>MMVISEKVRKALNDQLNREIYSSYLYLSMATYFDAEGFKGFAHWMKKQAQEELTHAMKFYEYIYERGGRVELEAIEKPPSNWNGIKDAFEAALKHEEFVTQSIYNILELASEEKDHATVSFLKWFVDEQVEEEDQVREILDLLEKANGQMSVIFQLDRYLGQRE[8x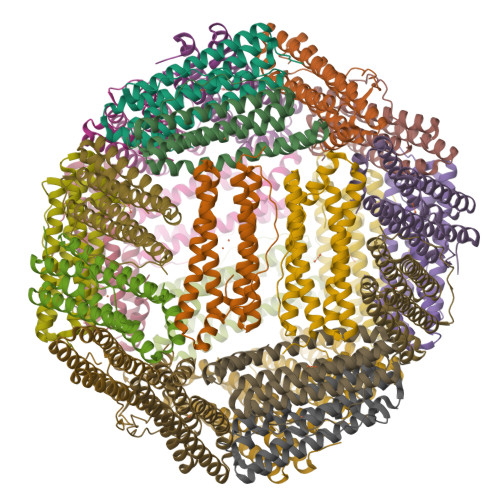]>[2x]MKFTVEREHLLKPLQQVSGPLGGRPT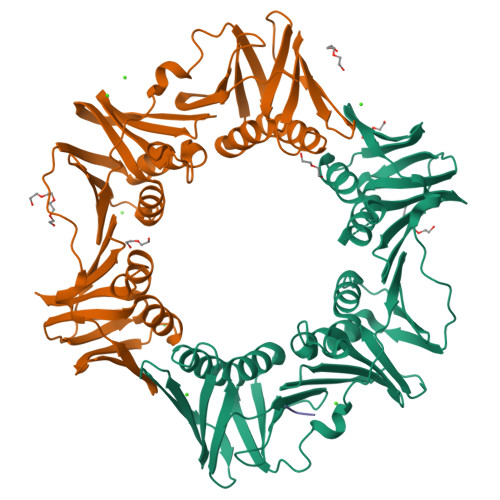LPILGNLLLQVADGTLSLTGTDLEMEMVARVALVQPHEPGATTVPARKFFDICRGLPEGAEIAVQLEGERMLVRSGRSRFSLSTLPAADFPNLDDWQSEVEFTLPQATMKRLIEATQFSMAHQDVRYYLNGMLFETEGEELRTVATDGHRLAVCSMPIGQSLPSHSVIVPRKGVIELMRMLDGGDNPLRVQIGSNNIRAHVGDFIFTSKLVDGRFPDYRRVLPKNPDKHLEAGCDLLKQAFARAAILSNEKFRGVRLYVSENQLKITANNPEQEEAEEILDVTYSGAEMEIGFNVSYVLDVLNALKCENVRMMLTDSVSSVQIEDAASQSAAYVVMPMRL;> ALDLF> MKIIITGEPGVGKTTLVKKIVERLGKRAIGFWTEEVRDPETKKRTGFRIITTEGKKKIFSSKFFTSK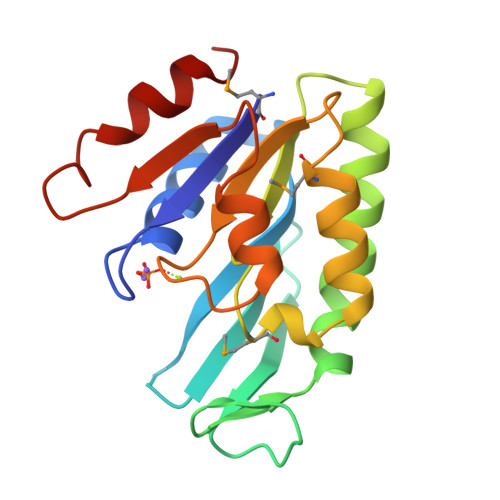KLVGSYGVNVQYFEELAIPILERAYREAKKDRRKVIIIDEIGKMELFSKKFRDLVRQIMHDPNVNVVATIPIRDVHPLVKEIRRLPGAVLIELTPENRDVILEDILSLLER> MTIEKEIEGLIHKTNKDLLNENANKDSRVFPTQRDLMAGIVSKHIAKNMVPSFIMKAHESGIIHVHDIDYSPALPFTNCCLVDLKGMLENGFKLGNAQIETPKSIGVATAIMAQITAQVASHQYGGTTFANVDKVLSPYVKRTYAKHIEDAEKWQIADALNYAQSKTEKDVYDAFQAYEYEVNTLFSSNGQTPFVTITFGTGTDWTERMIQKAILKNRIKGLGRDGITPIFPKLVMFVEEGVNLYKDDPNYDIKQLALECASKRMYPDIISAKNNKAITGSSVPVSPMGCRSFLSVWKDSTGNEILDGRNNLGVVTLNLPRIALDSYIGTQFNEQKFVELFNERMDLCFEALMCRISSLKGVKATVAPILYQEGAFGVRLKPDDDIIELFKNGRSSVSLGYIGIHELNILVGRDIGREILTKMNAHL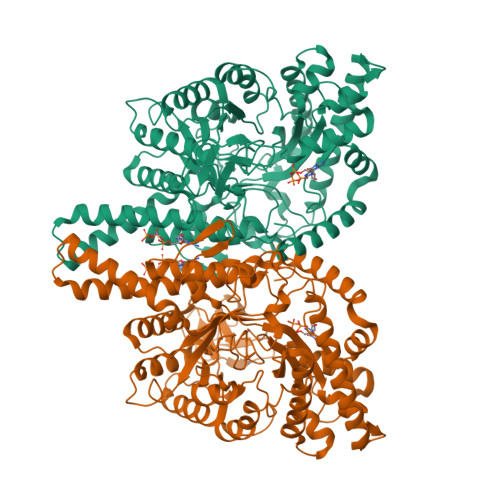KQWTERTGFAFSLYSTPAENLCYRFCKLDTEKYGSVKDVTDKGWYTNSFHVSVEENITPFEKISREAPYHFIATGGHISYVELPDMKNNLKGLEAVWDYAAQHLDYFGVNMPVDKCFTCGSTHEMTPTENGFVCSICGETDPKKMNTIRRTCAYLGNPNERGFNLGKNKEIMHRVKHQ> MRYRPVIGLEIHVQLSTKT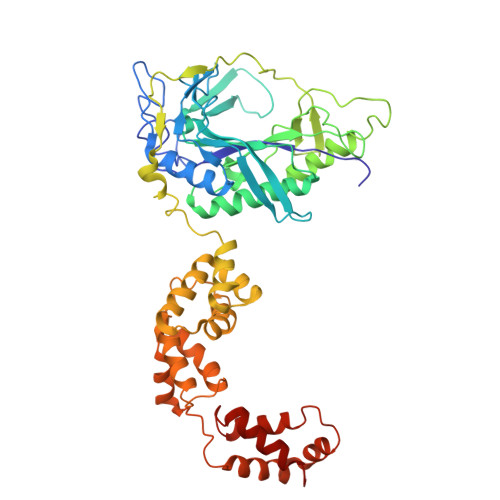KAFCSCPADVFELPPNTAICPVCTGQPGALPVPNEEMIRFAVKTALALNCKIHKYSRFDRKNYFYPDLPKGYQISQYFYPIATEGFLEIDGDEGRKKVRIRRLHLEEDAGKLVHEGDSITRASYSLVDMNRCGVPLIEIVTEPDISSPREARVFMEKLRSIVRYLGVSTGDMEKGALRCDANISVVDTETGRQSNRVEVKNMNSFRFVERALEYEFERIVKAMERGEDVERETRGWDMATKITVSMRGKEEESDYRYFPEPDIPPVVLSDEYLEEVKKELPELPDEKAERFMREYGLPEYDAKVLTSSKELAEFFEECVKVVNRPKDLSNWIMTEVLRELNERNIEITESKLTPQHFADLFKLMDEGKISIKIAKEIFPEVFETGKMPSQIVEEKGLTQINDEKLIEELVKKAMEQNPKAVQDYKSGKKKAAGFFVGYVMRETKGKANPELTNRIIQKLLEGE> MADNVAGNDRLIWIDLEMTGLDTDRDSIIEIATIVTDAQLNVLAEGPELA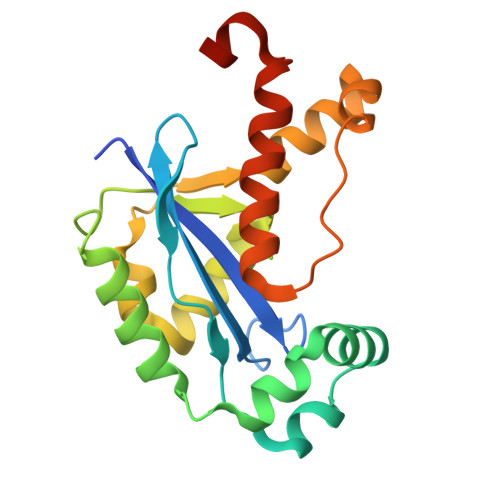IAHSLETLEAMDEWNRNQHRRSGLWQRVLDSQVTHAQAEAQTVAFLGEWIRAGASPMCGNSICQDRRFLHRQMSRLERYFHYRNLDVSTIKELARRWAPAVASGFAKSSAHTALSDVRDSIDELRHYRQFMGTLGGDNGGGVQN> MEPTSGFAEQPGPVKAESEEQEPAQWQALPVLSEQQSGAVELILAYAAPVLDKRQTSRLLREVSAVYPLPAQPHLKRVRPSRSAGGAQSSDLLLCLAGPSAGPRSLAELLPRPAVDPRGLGTPFLVPLPARPPLTRSQFEEARAHWPTSFHEDKQVTSALAGQLFSTQERAAMQTHMERAVCAAQRAAAQGLRAVGAVVVDPASDRVLATGHDCSSVASPLLHAVMVCIDLVAQGQGEDSL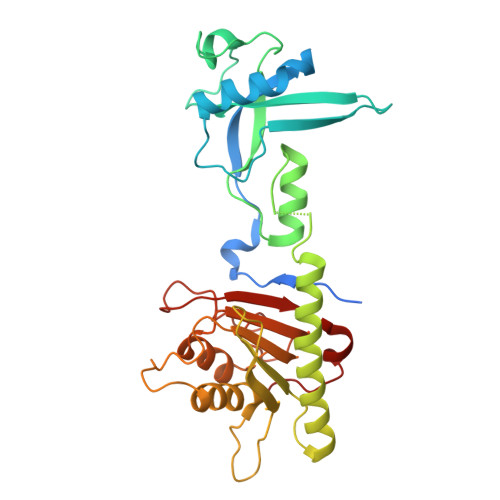PYVCTGYDLYVTREPCVMCAMALVHARIQRVFYGAPSPDGALGTLFRVHARPDLNHRFQVFRGILEDQCRQLDPDP> HINLKVAGQDGSVVQFK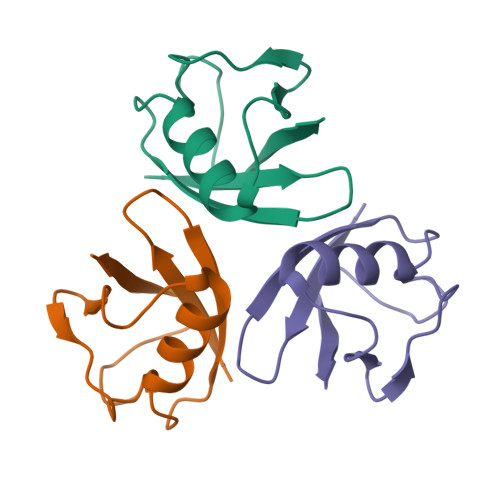IKRHTPLSKLMKAYCERQGLSMRQIRFRFDGQPINETDTPAQLEMEDEDTIDVFQ N-({4'-[(4-isobutyrylphenoxy)methyl]biphenyl-4-yl}sulfonyl)-D-valine | C28 H31 N O6 S | 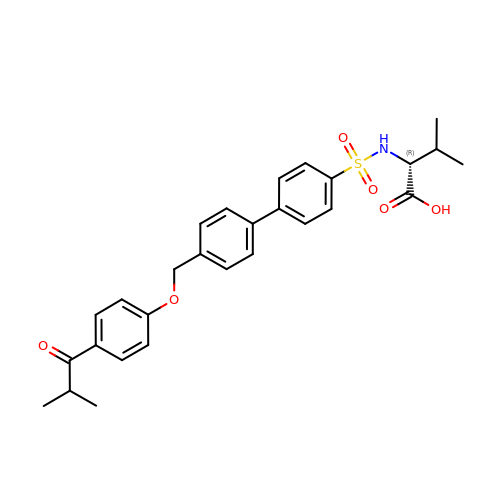JGTIIKHYSZFICL-AREMUKBSSA-N> KENA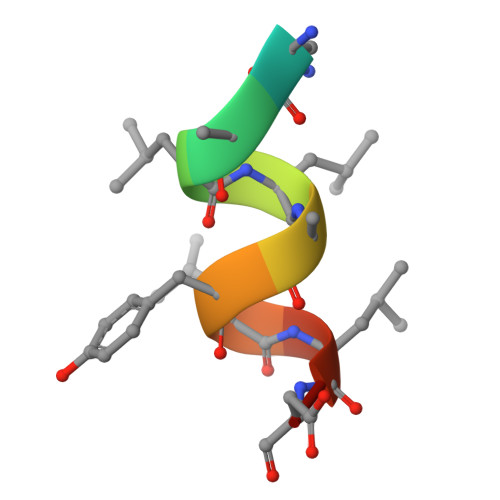LLRYLLDK>[4x]GSMKTNDNYIEEVTAKVLTSGKYSTLYPPTVRRVTERLFDRYPPKQLEKEVRKKLHQAYGAYIGGIDGKRLEKKIEKIIHEIPNPTTDEATRTEWEKEICLKILNLHTSTNERTVAYDELYQKIFEVTGVPTSITDAGCALNPFSFPFFTEAGMLGQYIGFDLDKGMIEAIEHSLRTLNAPEGIVVKQGDI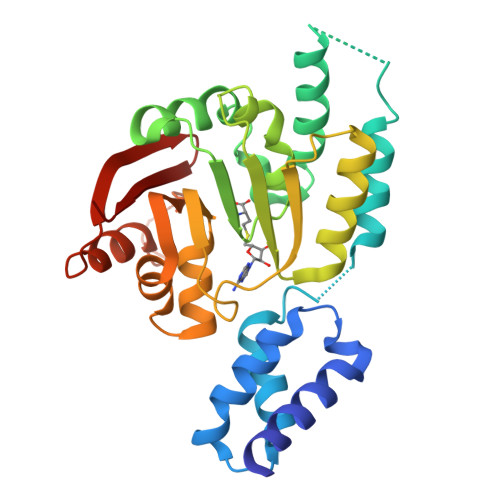LSDPSGESDLLLMFKLYTLLDRQEEASGLKILQEWKYKNAVISFPIKTISGRDVGMEENYTVKFENDLVGSDLRIMQKLKLGNEMYFIVSRL> AVAQ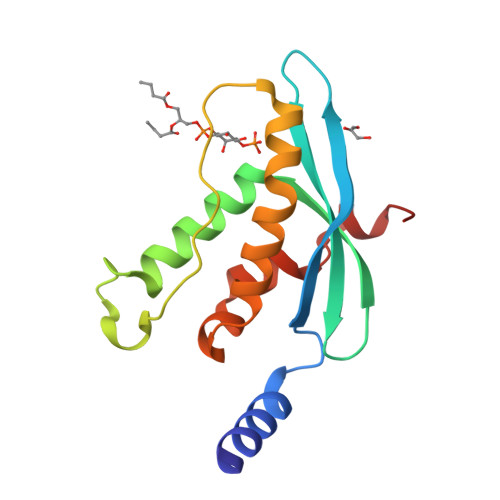QLRAESDFEQLPDDVAISANIADIEEKRGFTSHFVFVIEVKTKGGSKYLIYRRYRQFHALQSKLEERFGPDSKSSALACTLPTLPAKVYVGVKQEIAEMRIPALNAYMKSLLSLPVWVLMDEDVRIFFYQSPYDSEQVP> SMGESRVILAFGDSLFAGYGLDKGESYPAKLETALRSHGINARIINAGVSGDTTAAGLQRIKFVLDSQPDKPELAIVELGGNDLLRGLSPAEARQNLSGILEELQRRKIPILLMGMRAPPNLGAKYQREFDGIYPYLAEKYDAKLVPFFLEAVADRPDLIQKAHVHPTARGVEELVSATSNAVAKALPAKK

Here, we reported the enzymatic characterizations and crystal structures of marine bacterial esterases CrmE10 and AlinE4. The results showed that both CrmE10 and AlinE4 belong to the SGNH-hydrolase superfamily and the bacterial lipolytic enzyme GDSL family. The SGNH-hydrolase family, a superfamily that includes the bacterial lipolytic enzyme GDSL family, consists of enzymes possessing four strictly conserved residues, Ser, Gly, Asn, and His, in four conserved blocks, I, II, III, and V, respectively. Among these four residues, Ser and His serve as catalytic residues, and Ser, Gly, and Asn serve as oxyanion hole residues.

According to sequence alignment, the catalytic triad of CrmE10 consisted of Ser29, Asp178, and His181, and it was composed of Ser13, Asp162, and His165 in AlnE4. In mutants AlinE4-S13A, AlinE4-D162A, and AlinE4-H165A, catalytic activities toward p-NP esters were almost abolished. However, the function of the Asp residue was barely investigated. Although the mutant AlinE4-D162A did not show significant variation compared with wild-type AlinE4, the B-factor of this loop was lower than wild-type AlinE4. In addition, one key residue (Asp162 in AlinE4/Asp178 in CrmE10) was found to be able to stabilize the conformation of both esterases and the metal ion Cd2+ reduced enzymatic activity by blocking proton transfer and substrate binding.> TNWYANL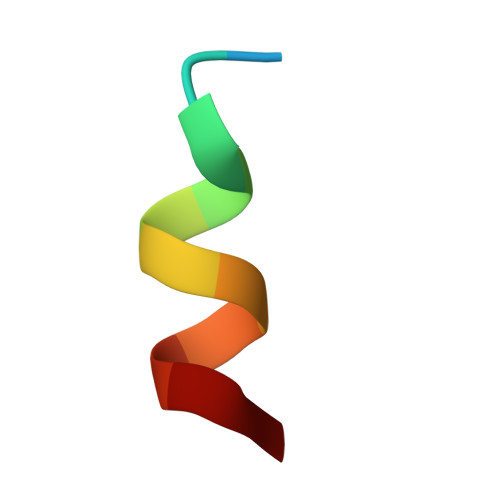EKLLR>MGGSHHHHHHGDDDDKMTKTFKTLDDFLGTHFIYTYDNGWEYEWYAKNDHTVDYRIHGGMVAGRWVTDQKADIVMLTEGIYKISWTEPTGTDVALDFMPNEKKLHGTIFFPKWVEEHPEITVTYQNEHIDLME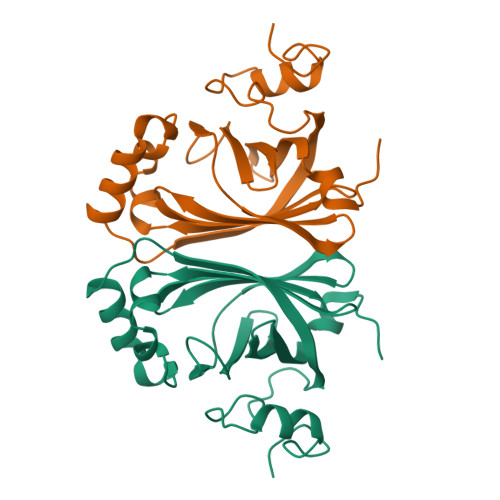QSREKYATYPKLVVPEFANITYMGDAGQNNEDVISEAPYKEMPNDIRNGKYFDQNYHRLNK[2x]>[2x]MAGNFSEIESQGNISLKFGFLGLGMGGCAIAAECANKETQIKNNKYPYRAILVNTNSQDFNKIEIKNTGNVRKIQLEGYEQGAARNPQVGEEAFVKHETKIFEAVKQEFEDRDFIWITCGLGGGTGTGALLKAIEMLYEHDYNFGLLLTLPRD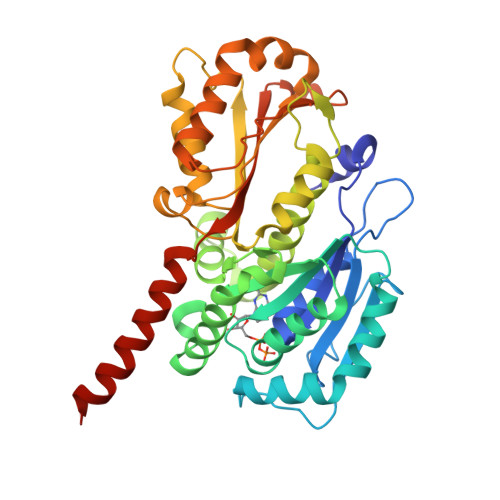AEALKVLENATSRIRSIAMNQEAFGSIVLIDNAKLYRKFEEENPSALANEYTSYSNKYIADALHEINLVTSSFTPFSDTHFDASEFAQVINTPGVLSLAKLELKSNQLDTENPLGYLTQLGNALEKGVLYDTEREELESAKKSALSIVTSPLRAGRLYNFSFLNQMENFLKERTPYVDERPIAPYVNKHTTKKEEDIVKFYSVVAGLPLPKRVSDIIDEITRIKEEREQANSKKSN>GPYASLTEIEHLVQSVCKSYRETCQLRLEDLLRQRSNIFSREEVTGYQRKSMWEMWERCAHHLTEAIQYVVEFAKRLSGFMELCQNDQIVLLKAGAMEVVLVRMCRAYNADNRTVFFEGKYGGMELFRALGCSELISSIFDFSHSLSALHFSEDEIALYTALVLINAHRPGLQEKRKVEQLQYNLELAFHHHLSKTHRQSILAKLPPKGKLRSLCSQHVERLQIFQHLHPIVVQAAFPPLYKELFSTETESPVGLSK[4x];>[4x]NSHQKVTLLQLL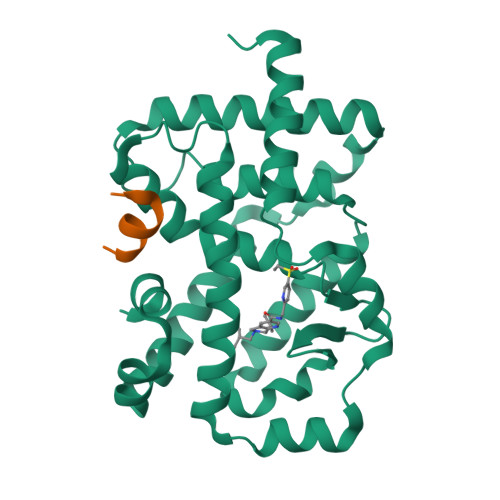LGHKNEEN N'-[(1S,2S)-2-[(4S)-1-benzyl-5-oxoimidazolidin-4-yl]-1-(3,5-difluorobenzyl)-2-hydroxyethyl]-5-methyl-N,N-dipropylbenzene-1,3-dicarboxamide 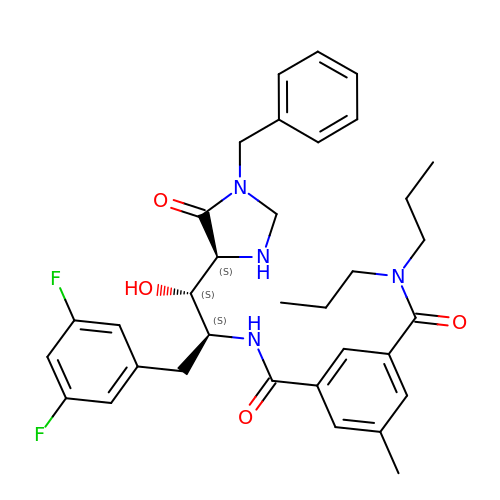| C34 H40 F2 N4 O4 | HZWNNIVRFLRAQW-CHQNGUEUSA-N>[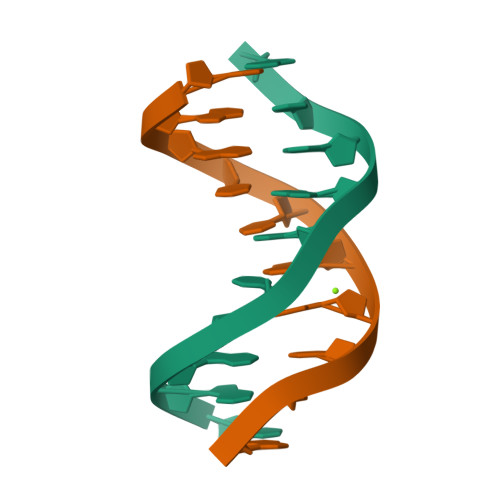2x]CGATTAATCG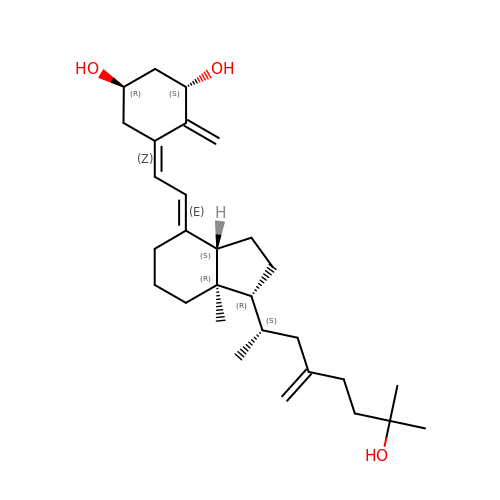(1~{R},3~{S},5~{Z})-5-[(2~{E})-2-[(1~{R},3~{a}~{S},7~{a}~{R})-7~{a}-methyl-1-[(2~{S})-7-methyl-4-methylidene-7-oxidanyl-octan-2-yl]-2,3,3~{a},5,6,7-hexahydro-1~{H}-inden-4-ylidene]ethylidene]-4-methylidene-cyclohexane-1,3-diol | C29 H46 O3 | LVXRHQNFZLEICU-LIOGGTHJSA-N>[4x]MEPSALRKAGSEQEEGFEGLPRRVTDLGMVSNLRRSNSSLFKSWRLQCPFGNNDKQESLSSWIPENIKKKECVYFVESSKLSDAGKVVCQCGYTHEQHLEEATKPHTFQGTQWDPKKHVQEMPTDAFGDIVFTGLSQKVKKYVRVSQDTPSSVIYHLMTQHWGLDVPNLLISVTGGAKNFNMKPRLKSIFRRGLVKVAQTTGAWIITGGSHTGVMKQVGEAVRDFSLSSSYKEGELITIGVATWGTVHRREGLIHPTGSFPAEYILDEDGQGNLTCLDSNHSHFILVDDGTHGQYGVEIPLRTRLEKFISEQTKERGGVAIKIPIVCVVLEGGPGTLHTIDNATTNGTPCVVVEGSGRVADVIAQVANLPVSDITISLIQQKLSVFFQEMFETFTESRIVEWTKKIQDIVRRRQLLTVFREGKDGQQDVDVAILQALLKASRSQDHFGHENWDHQLKLAVAWNRVDIARSEIFMDEWQWKPSDLHPTMTAALISNKPEFVKLFLENGVQLKEFVTWDTLLYLYENLDPSCLFHSKLQKVLVEDPERPACAPAAPRLQMHHVAQVLRELLGDFTQPLYPRPRHNDRLRLLLPVPHVKLNVQGVSLRSLYKRSSGHVTFTMDPIRDLLIWAIVQNRRELAGIIWAQSQDCIAA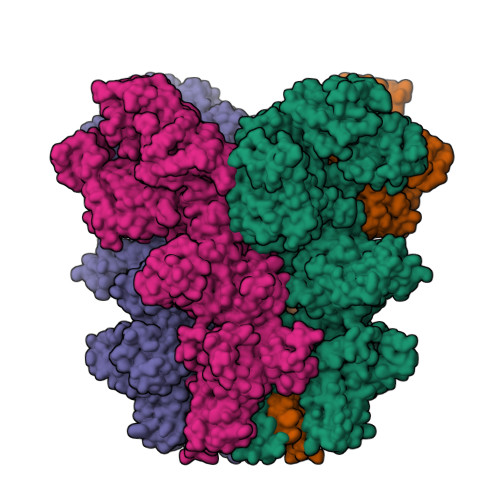ALACSKILKELSKEEEDTDSSEEMLALAEEYEHRAIGVFTECYRKDEERAQKLLTRVSEAWGKTTCLQLALEAKDMKFVSHGGIQAFLTKVWWGQLSVDNGLWRVTLCMLAFPLLLTGLISFREKRLQDVGTPAARARAFFTAPVVVFHLNILSYFAFLCLFAYVLMVDFQPVPSWCECAIYLWLFSLVCEEMRQLFYDPDECGLMKKAALYFSDFWNKLDVGAILLFVAGLTCRLIPATLYPGRVILSLDFILFCLRLMHIFTISKTLGPKIIIVKRMMKDVFFFLFLLAVWVVSFGVAKQAILIHNERRVDWLFRGAVYHSYLTIFGQIPGYIDGVNFNPEHCSPNGTDPYKPKCPESDATQQRPAFPEWLTVLLLCLYLLFTNILLLNLLIAMFNYTFQQVQEHTDQIWKFQRHDLIEEYHGRPAAPPPFILLSHLQLFIKRVVLKTPAKRHKQLKNKLEKNEEAALLSWEIYLKENYLQNRQFQQKQRPEQKIEDISNKVDAMVDLLDLDPLKRSGSMEQRLASLEEQVAQTAQALHWIVRTLRASGFSSEADVPTLASQKAAEEPDAEPGGRKKTEEPGDSYHVNARHLLYPNCPVTRFPVPNEKVPWETEFLIYDPPFYTAERKDAAAMDPMGDTLEPLSTIQYNVVDGLRDRRSFHGPYTVQAGLPLNPMGRTGLRGRGSLSCFGPNHTLYPMVTRWRRNEDGAICRKSIKKMLEVLVVKLPLSEHWALPGGSREPGEMLPRKLKRILRQEHWPSFENLLKCGMEVYKGYMDDPRNTDNAWIETVAVSVHFQDQNDVELNRLNSNLHACDSGASIRWQVVDRRIPLYANHKTLLQKAAAEFGAHY>[2x]SNAMPLPKSLKYGD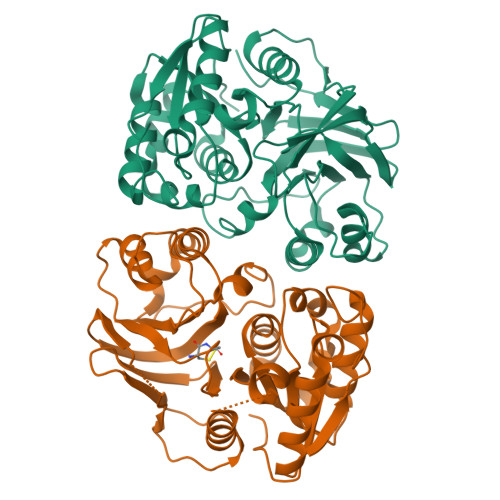TIGIYSPSSPVTYTSPKRFERAKSYLLQKGFHILEGSLTGRYDYYRSGSIQERAKELNALIRNPNVSCIMSTIGGMNSNSLLPYIDYDAFQNNPKIMIGYSDATALLLGIYAKTGIPTFYGPALVPSFGEFEPFVDDTYKYFLETLLHDQALPYNIKQPLFWSDEFINAEEKTKEKELRPNNWISVTNGQATGRVIGGNLNTIQGIWGSPYMPCIQEGDILFIEDSSKDAATIERSFSFLKINGVFDKVSGIILGKHEQFDDCGTNRKPYEILLEVLQNQRIPLLADFDCCHTHPMITMPIGVQVKMDATNKTIHILEKWKI>[2x]SMNPTAEEVLSWSQNFD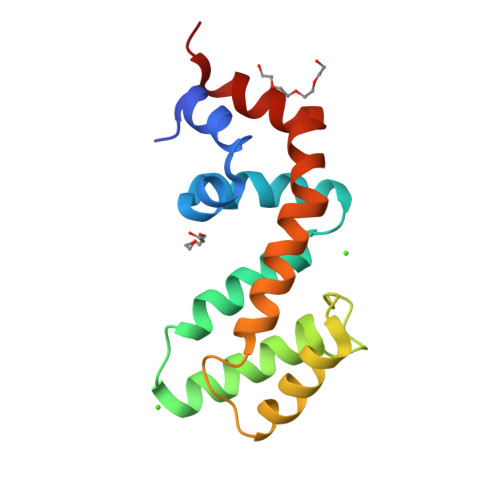KMMKAPAGRNLFREFLRTEYSEENLLFWLACEDLKKEQNKKVIEEKARMIYEDYISILSPKEVSLDSRVREVINRNLLDPNPHMYEDAQLQIYTLMHRDSFPRFLNSQIYKSFVESTAGS Glutaminase catalyzes the first step of glutamine metabolism, converting glutamine to glutamate, which enters the tricarboxylic acid cycle. In human, glutaminase is encoded by two different genes, GLS1 and GLS2.1 GLS1 can be alternatively spliced into kidney glutaminase A (KGA) and highly active glutaminase isoform C (GAC)1. Glutaminase, especially the GAC isoform, is highly overexpressed in various cancers for the utilization of glutamine. GAC can be further activated by anions. It has been observed that GAC can form active filaments both in vitro and in vivo.

Cryo-EM samples of GAC containing Pi and an analog of glutamine, 6-Diazo-5-oxo-L-norleucine (DON) were prepared. We resolved the structure of GAC filament at a resolution of 2.9 Å. GAC forms filaments with tetramers as the helical unit. By viewing the filament from the top, the twist angle of ~51° can be observed. A GAC tetramer contains four Pi binding sites, which are located on the dimer–dimer interface, consisting of R317 and K320 on the activation loop (AL), as well as R387, Y394′ and K398′ on the dimer–dimer interface. Significant conformational changes were observed in the GAC tetramer bound with Pi when comparing the tetramers in filament to free tetramers, and the RMSD between them is greater than 2 Å. First, the GAC-PF tetramer changes into a compressed form, with each protomer rotating by 5.6°. Second, the AL (residues 308–334) of each protomer in the GAC-PF tetramer is reshaped and stabilized. However, in the GAC-PF tetramer, the B-factor analysis of our models shows that the AL is in a stable state. However, when Pi-bound GAC forms a filament, the AL is stabilized, and the pocket is remodeled, resulting in highly active GAC.

>LVASGENKIKQGLLPSLEDLLFYTIAEGQEKIPVHKFITALKSTGLRTSDPRLKECMDMLRLTLQTTSDGVMLDKDLFKKCVQSNIVLLTQAFRRKFVIPDFMSFTSHIDELYESAKKQSGGKVADYIPQLAKFSPDLWGVSVCTVDGQRHSTGDTKVPFCLQSCVKPLKYAIAVNDLGTEYVHRYVGKEPSGLRFNKLFLNEDDKPHNPMVNAGAIVVTSLIKQGVNNAEKFDYVMQFLNKMAGNEYVGFSNATFQSERESGDRNFAIGYYLKEKKCFPEGTDMVGILDFYFQLCSIEVTCESASVMAATLANGGFCPITGERVLSPEAVRNTLSLMHSCGMYDFSGQFAFHVGLPAKSGVAGGILLVVPNVMGMMCWSPPLDKMGNSVKGIHFCHDLVSLCNFHNYDNLRHFAKKLDPRREGGDQRHSFGPLDYESLQQELALKETVWKKVSPESNEDISTTVVYRMESLGEKS[4x]> IVGGYTCGANTVPYQVSLNSGYHFCGGSLINSQWVVSAAHCYKSGIQVRLGEDNINVVEGNEQFISASKSIVHPSYNSNTLNNDIMLIKLKSAASLNSRVASISLPTSCASAGTQCLISGWGNTKSSGTSYPDVLKCLKAPILSDSSCKSAYPGQITSNMFCAGLEGGDSCQGDSGGPVVCSGKLQGIVSWGSGCAKNKPGVYTKVCNYVSWIKQTIASN;> SALYAPSALVLT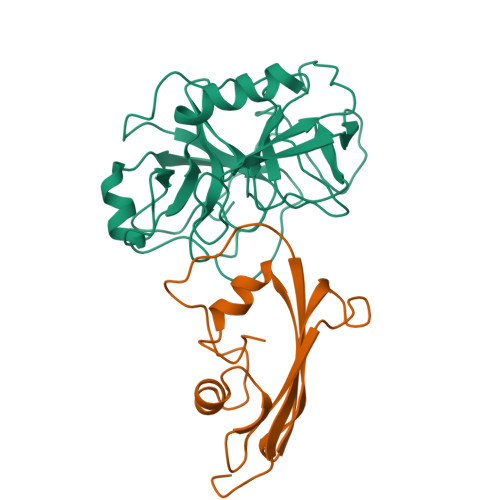VGKGVSATTAAPERAVTLTCAPGPSGTHPAAGSACADLAAVGGDLNALTRGEDVGCPKVYDPVLLTVDGVWQGKRVSYERVFSNECEMNAHGSSVFAF>GSHMATPWSGYLDDVSAKFDTGVDNLQTQVTEALDKLAAKPSDPALLAAYQAKLSEYNLYRNAQSNTVKVFKDIDAAIIQNFR[20x]

Salmonella enterica serovar Typhimurium (S. Typhimurium), a gram-negative bacterium responsible for innumerable cases of acute gastroenteritis worldwide, utilizes two T3SSs, encoded within its pathogenicity islands 1 (SPI-1) and 2 (SPI-2), to invade cells and establish an intracellular replicative niche. The core component of this machine is the envelope-associated needle complex, which consists of a multiring base, an inner rod, and a needle filament extension that protrudes several nanometers from the bacterial surface. The entire structure is traversed by an approximately 2-nm channel that serves as a conduit for the T3SS protein substrates as they pass through the bacterial envelope. Furthermore, four residues at the end of the C-terminal α-helix, three charged (K66, D70, and R80) and one polar uncharged (Q77), form the lumen of the channel and create an electrostatic surface potential of alternating charges, which spiral upwardly about the needle, a feature that has been proposed to be important for substrate translocation.

Since we observed no differences between the structures of in vivo and in vitro polymerized needle filaments, we solved the cryo-EM structures of PrgIS49A and PrgIV67A filaments assembled in vitro from purified mutant proteins. These mutants are located within the C-terminal α-helix and resulted in specific phenotypes, such as constitutive secretion (PrgIS49A) or deficiency in the secretion of SipB (PrgIV67A). We found that S. Typhimurium strains expressing the PrgI mutants D10A, D11A, V20A, S49A, E53A, N55A, R58A, N63A, and N78A retained the ability to display SipD at the tip of the needle filament. Although limited by the resolution, the differences in helical symmetry in the two mutants analyzed resulted in small but measurable local differences in the distance between the mutated residues and neighboring residues from adjacent PrgI subunits in the assembled filaments. However, no significant difference among PrgIWT, PrgIS49A, and PrgIV67A was detected in the structures of the monomers extracted from the assembled filaments, with a Cα RMSD over 77 residues of 0.152 Å between PrgIWT and PrgIS49A and 0.225 Å between PrgIWT and PrgIV67A. However, the predicted electrostatic potential of the lumens of filaments assembled with the PrgIS49A and PrgIV67A mutants showed significant differences with wild type. Taken together, these results indicate that the PrgI mutations resulted in defined structural changes altering the surface properties of the lumen, which may be responsible for the phenotypes observed in bacteria expressing these mutant filament proteins. Indeed, the two mutants analyzed by this approach showed subtle but distinct changes on the electrostatic properties of the lumen surface even though the mutated residues do not directly participate in configuring the lumen surface.> MSMSNYQTLVDVNNAMNKMLRAYVNEAVAIRFDLPDVDATQADAAISVFLYDIHEDLQLRTAESRGFNAGAGRLLPGWVNVKCNYLITYWESTGPATDADNPDSQ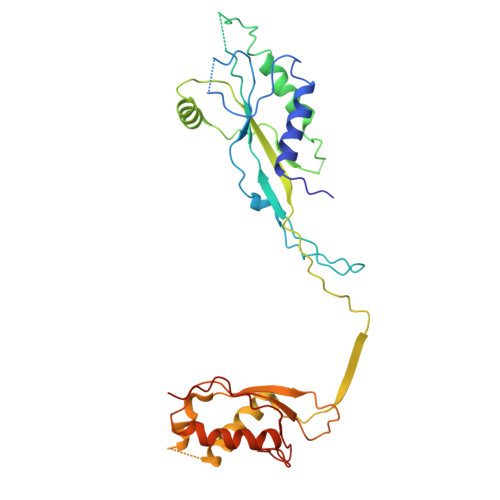PDNQAIQVMSQVLAALINNRQLADIPGAYTQVMPPKENLNSLGNFWQSLGNRPRLSLNYCVTVPISLSDKGEEMTPVKSLSTTVEPKAPLSPLVITDALREQLRVALGGDYDACLAMTHVNLDSSPVANSDGSAAEIRVSLRVYGMTPTEYLAPMNTVFNEWEKSEAAAVTPDGYRVYINAVDKTDLTGI> GPLGSSSGQSNNNSDTCAEFRIKYVGAIEKLKLSEGKGLEGPLDLINYIDVAQQDGKLPFVPPEEEFIMGVSKYGIKVSTSDQYDVLHRHALYLIIRMVCYDDGLGAGKSLLALKTTDASNEEYSLWVYQCNSLEQAQAICKVLSTAF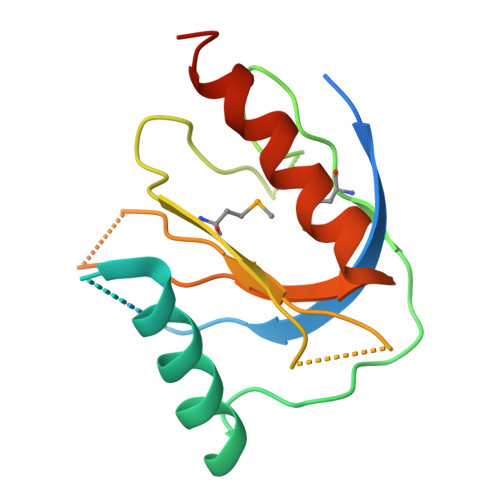DSVLTSEKP> MTTSQKHRDFVAEPMGEKPVGSLAGIGEVLGKKLEERGFDKAYVVLGQFLVLK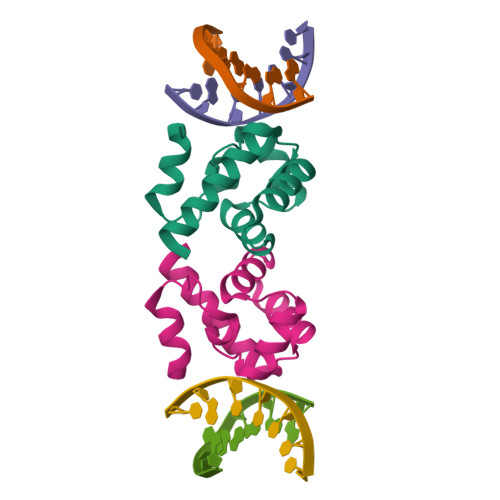KDEDLFREWLKDTCGANAKQSRDCFGCLREWCDAFL>THMRCRVYYEDTDSEGVVYHANYLKYCERARSEFFFKQNVLPENEEGVFVIRSI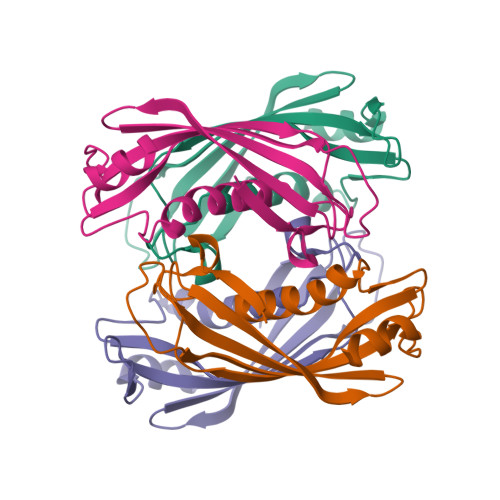KADFFTPASLGQVLEIRTQIKELRKVFVVLFQEIYCIQNASLEPMKPFKVFASEIKFGFVNRSTYSPIAIPKLFKELLNAI[4x]> SSEKLFRIQCGYQNYDWGKIGSSSAVAQFVHNSDPSITIDETKPYAELWMGTHPSVPSKAIDLNNQTLRDLVTAKPQEYLGESIITKFGSSKELPFLFKVLSIEKVLSIQAHPDKKLG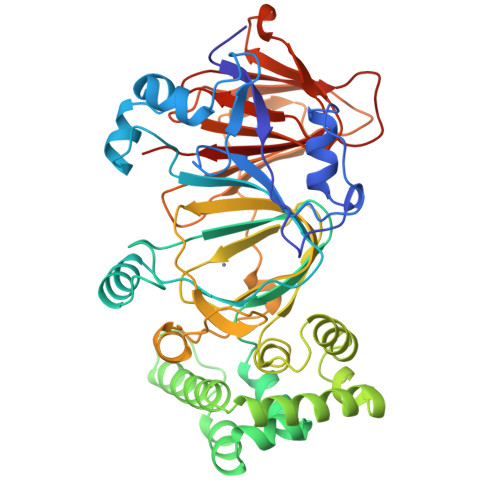AQLHAADPKNYPDDNHKPEMAIAVTDFEGFCGFKPLDQLAKTLATVPELNEIIGQELVDEFISGIKLPAEVGSQDDVNNRKLLQKVFGKLMNTDDDVIKQQTAKLLERTDREPQVFKDIDSRLPELIQRLNKQFPNDIGLFCGCLLLNHVGLNKGEAMFLQAKDPHAYISGDIIECMAASDNVVRAGFTPKFKDVKNLVEMLTYSYESVEKQKMPLQEFPRSKGDAVKSVLYDPPIAEFSVLQTIFDKSKGGKQVIEGLNGPSIVIATNGKGTIQITGDDSTKQKIDTGYVFFVAPGSSIELTADSANQDQDFTTYRAFVEA Synaptic vesicle glycoprotein 2a (SV2A), a putative membrane transporter in the synaptic vesicles (SVs), has been identified as a target of LEV and BRV. SV2A also serves as a receptor for botulinum neurotoxin (BoNT), which is the most toxic protein and has paradoxically emerged as a potent reagent for therapeutic and cosmetic applications. SV2 family proteins belong to the major facilitator superfamily (MFS) with 12 predicted transmembrane helices. In addition to the transmembrane domain (TMD) core, a cytosolic N-terminal region and a large fourth luminal domain (LD4) are present.

The open edge of the β-strand from the β-hairpin of HCA2 forms backbone hydrogen bonding interactions with the open edge of the C-terminal β-strand from the β-helix structure of LD4A. In addition to the backbone–backbone interaction, the SV2A His578 side chain forms a salt bridge with the BoNT/A2 Glu1156 side chain. SV2A Phe576 contributes to the van der Waals interactions with Ser1142 and Val1144 of BoNT/A2. The protein–protein interaction between HCA2 and LD4A creates a relatively small binding interface with a buried surface area of 464 Å2. To enhance this interaction, N-glycans attached to LD4A contribute to binding. Three putative N-glycan sites, Asn498, Asn548, and Asn573 in SV2A, are mapped on LD4A. A N-glycan containing two N-acetylglucosamines (NAG)s and fucose (FUC) attached to Asn573 forms extensive contacts with HCA2. The BoNT/A2 Phe953 and the aliphatic portion of the BoNT/A2 Arg1064 form the van der Waals contacts with the two NAGs attached to LD4A.

> YASRTKVFPGERVEHVTFNFTLENQIHRGGQYFNDKFIGLRLKSVSFEDSLFEECYFEDVTSSNTFFRNCTFINTVFYNTDLFEYKFVNSRLINSTFLHNKEGCPLDVTGT;> KNIVNTSILSIVYKKDDLIDLSRYGAKINIGDRVYYDSIDKNQIKLINLESSTIEVILKNAIVYNSMYENFSTSFWIKIPKYFSKINLNNEYTIINCIENNSGWKVSLNYGEIIWTLQDNKQNIQRVVFKYSQMVNISDYINRWIFVTITNNRLTKSKIYINGRLIDQKPISNLGNIHASNKIMFKLDGCRDPRRYIMIKYFNLFDKELNEKEIKDLYDSQSNSGILKDFWGNYLQYDKPYYMLNLFDPNKYVDVNNIGIRGYMYLKGPRGSVVTTNIYLNSTLYEGTKFIIKKYASGNEDNIVRNNDRVYINVVVKNKEYRLATNASQAGVEKILSALEIPDVGNLSQVVVMKSKDDQGIRNKCKMNLQDNNGNDIGFIGFHLYDNIAKLVASNWYNRQVGKASRTFGCSWEFIPVDDGWGESSL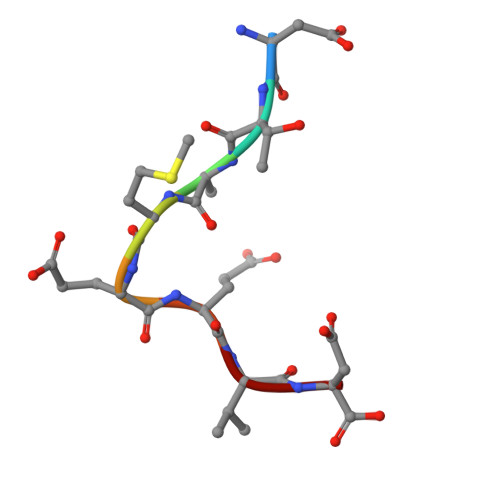> DTEMEEVD>[2x]TAPSQVLKIRRPDDWHLHLRDGDMLKTVVP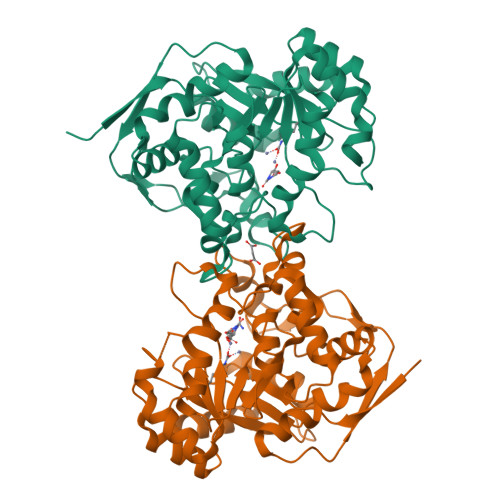YTSEIYGRAIVMPNLAPPVTTVEAAVAYRQRILDAVPAGHDFTPLMTCYLTDSLDPNELERGFNEGVFTAAKLYPANATANSSHGVTSVDAIMPVLERMEKIGMPLLVHGEVTHADIDIFDREARFIESVMEPLRQRLTALKVVFEHITTKDAADYVRDGNERLAATITPQHLMFNRNHMLVGGVRPHLYCLPILKRNIHQQALRELVASGFNRVFLGTDSAPHARHRKESSCGCAGCFNAPTALGSYATVFEEMNALQHFEAFCSVNGPQFYGLPVNDTFIELVREEQQVAESIALTDDTLVPFLAGETVRWSVKQ> ADKELKFLVVDDFSTMRRIVRNLLKELGFNNVEEAEDGVDALNKLQAGGYGFVISDWNMPNMDGLELLKTIRADGAMSALPVLMVTAEAKKENVIAAAQAGASGY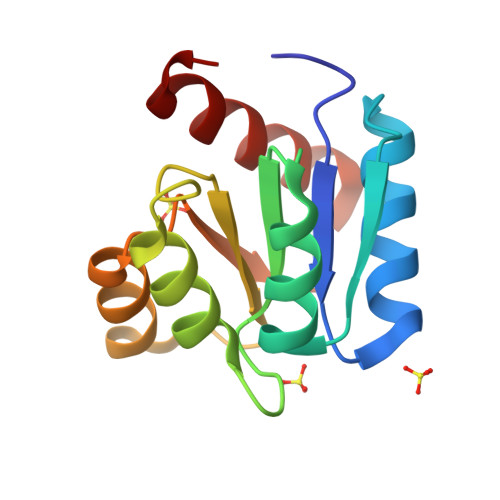VVKPFTAATLEEKLNKIFEKLGM> GSHMGKSMENVAMPVVDSENVSVVKKFYETDAAKEEKEAALVTYNNTYSLSKGIDLAEKDGKDFDVSASLSGTVVKAEKDPVLGYVVEVEHADGLSTVYQSLSEVSVEQGDKVKQNQVIGKSGKNLYSEDSGNHVHFEIRKD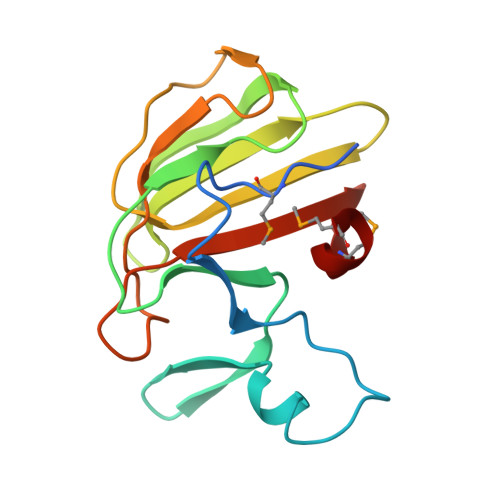GVAMNPLNFM> GLDTIPTTYVDAGSVFGKTGDAEKVLNGGWNYLMETFNSYANPGYGAMLRANDAMGSDVVLNSKYGFRTHNEFSAIYGKGGTNTLSWLLAYRVINDCNGVLDNIDAAEGTQADRNRIKGQALALRGFLYLHLASCYSFAIDKDPDAVCAPIYTQSTDETIAAEGKPASSVSEVYAQSINDLEEALELIPETYVRDAKHKIDNEVVLGILSRACLYARQWEKAKTYSDKLLAKDNYLMTESEYKAGFNSVDNKEWIWGHAQTNDQSNASYQFHYLDTTTKGSYYYSFNVDPYFRDLFEDGDYRKEMLFWATDPGADVESAAYVWMRNSKFRFRDI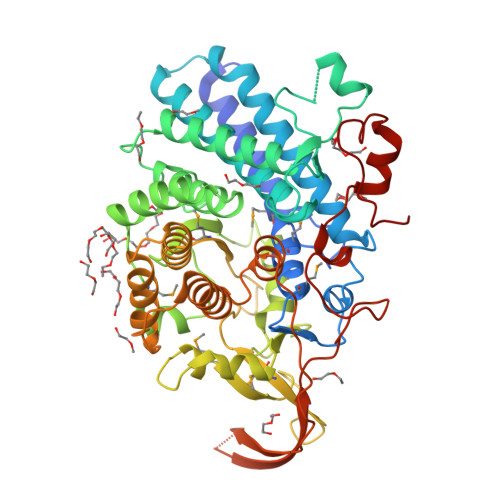ENQLGDIVLMRVAEIYLINAEAKAHLNDPDAINKLNDLKTARGAKTIHTNLSQQDLLETIWLERRKELWGEGFSLIDIIRNQQTVVRNAYPEGPIDYIYTDENGQTHTLKKKTQGHRFFNFPDKSAFCPNSKYYLYRITDSEELANKNLYKDHPKLSIYTK> MRNLMRCLIMIKSLIKGVDMSRKLAKTRILGYGLMICFLAGCFHPPYNNFQPDRRAVKRVGVDTGIGAVAGAIASGTASGTLIGAAAGGTVGLVASIYRDSKRKIIRDLQKQDIQYVEYGDTRTLIIPTDKYFMFSSPRLNEICYPGLNNVIRLLNFYPQSTIYVAGFTDNVGSRSHKRKLSQAQA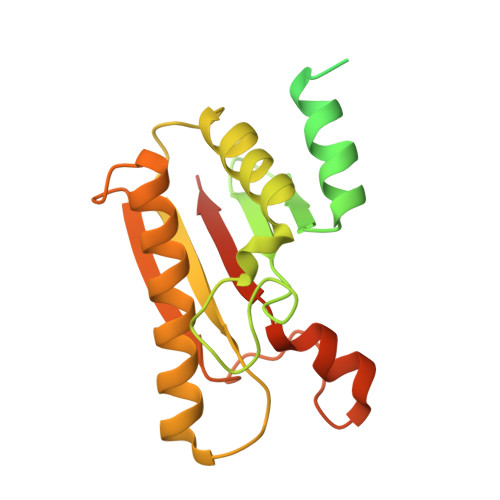ETMMTFLWANGIAAKRLKAEGYGDKNAISDNAIIHGSAQNRRIEIQWFTSPAQPPQPQMAYVK>KHGPLHPIPNRPVLTRARASLPLVLYIDRFLGGVFSKRRIPKRTQFGPVEGPLVRGSELKDCYIHLKVSLDKGDRKERDLHEDLWFELSDETLCNWMMFVRPAQNHLEQNLVAYQYGHHVYYTTIKNVEPKQELKVWYAASYAEFVN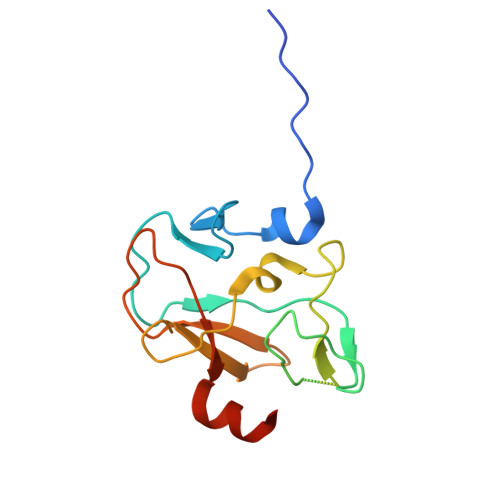QKIHD[4x]>[2x]MIINNL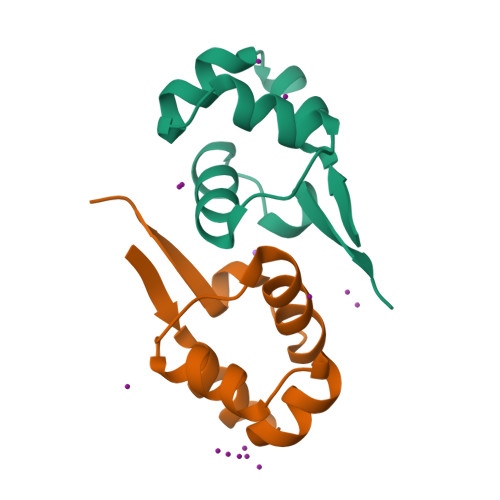KLIREKKKISQSELAALLEVSRQTINGIEKNKYNPSLQLALKIAYYLNTPLEDIFQWQPE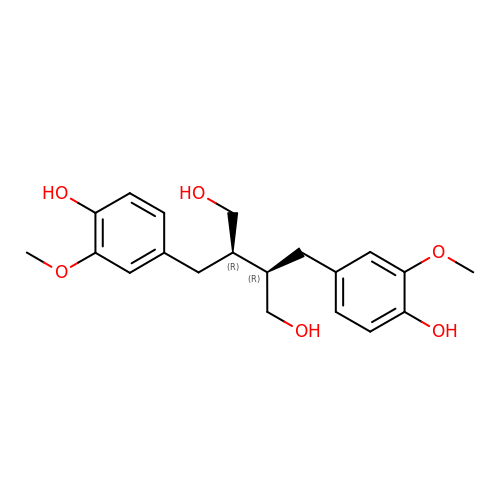(2R,3R)-2,3-bis[(3-methoxy-4-oxidanyl-phenyl)methyl]butane-1,4-diol | C20 H26 O6 | PUETUDUXMCLALY-HOTGVXAUSA-N> MDGTAAEPRPGAGSLQHAQPPPQPRKKRPEDFKFGKILGEGSFSTVVLARELATSREYAIKILEKRHIIKENKVPYVTRERDVMSRLDHPFFVKLYFTFQDDEKLYFGLSYAKNGELLKYIRKIGSFDETCTRFYTAEIVSALEYLHGKGIIHRDLKPENILLNEDMHIQITDFGTAKV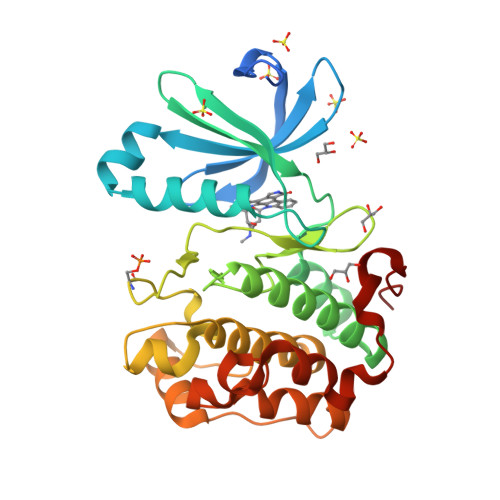LSPESKQARANSFVGTAQYVSPELLTEKSACKSSDLWALGCIIYQLVAGLPPFRAGNEYLIFQKIIKLEYDFPEKFFPKARDLVEKLLVLDATKRLGCEEMEGYGPLKAHPFFESVTWENLHQQTPPKLTA> AGAQDFVPHTADLAELAAAAGECRGCGLYRDATQAVFGAGGRSARIMMIGEQPGDKEDLAGLPFVGPAGRLLDRALEAADIDRDALYVTNAVKHFKFTRAAGGKRRIGKTPSRTEVVACRPWLIAEMTSVEPDVVVLLGATAAKALLGNDFRVTQHRGEVLHVDDVPGDPALVATVHPSSLLRGPKEERESAFAGLVDDLRVAADV

UdgX excises uracil from uracil-containing DNA to concurrently form a covalent bond with the resulting AP-DNA. Structurally, UdgX is highly similar to family-4 UDGs (F4-UDGs). However, UdgX is unique in possessing a flexible R-loop (105KRRIH109). Our earlier studies allowed us to propose a reaction mechanism of UdgX, which involves the formation of a covalent bond between H109 of UdgX with the C1′ position of the target deoxyribose sugar concurrently with the uracil excision from this site in DNA.

Substitutions of His109 in MsmUdgX with Ser, Gly, Ala, Gln, Cys and Lys showed the loss of its covalent complex formation with DNA but gained canonical UDG activities. We note that smaller and hydrophilic amino acid substitutions at His109, such as Gly or Ser showed higher Kcat/Km values. However, to better understand the mechanism of uracil excision by the H109 mutants, we determined their structures along with a pentameric DNA, TTUTT by X-ray crystallography. The DNA backbone could not be modelled into the experimental electron density map in any of the mutant structures that were determined. Nonetheless, all structures revealed the excised uracil and the side chain substitutions at position 109. The structures also revealed invariant interactions of N91 and H178 with uracil. When we arranged the mutants in the order of increasing cavity sizes (left), we noted that the canonical UDG activity of the mutants increased with their increasing cavity sizes to begin with and then with a further increase in the cavity size, the UDG activity declined (right). It suggested that the initial increase in UDG activity (H109K to H109Q to H109G) occurred because of the efficiency with which the water molecule could be localized to make a nucleophilic attack on the C1′ position. Interestingly, G109 the smallest amino acid substitution of H109 showed lower cavity volume than Ser, Cys or Ala due to an overall structural change near the active site.>[16x]SMELYNIKYAIDPTNKIVIEQVDNVDAFVHILEPGQE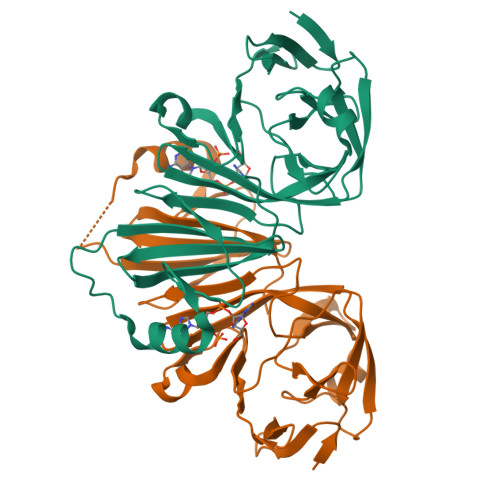VFDETLSQYHQFPGVVSSIIFPQLVLNTIISVLSEDGSLLTLKLENTCFNFHVCNKRFVFGNLPAAVVNNETKQKLRIGAPIFAGKKLVSVVTAFHRVGENEWLLPVTGIREASQLSGHMKVLNGVRVEKWRPNMSVYGTVQLPYDKIKQHALEQENKTPNALESCVLFYKDSEIRITYNKGDYEIMHLRMPGPLIQPNTIYYS>[4x]MEFKLQELNLTNQDTGPYGITVSDKGKVWITQHKANMISCINLDGKITEYPLPTPDAKVMCLTISSDGEVWFTENAANKIGRITKKGIIKEYTLPNPDSAPYGITEGPNGDIWFTEMNGNRIGRIT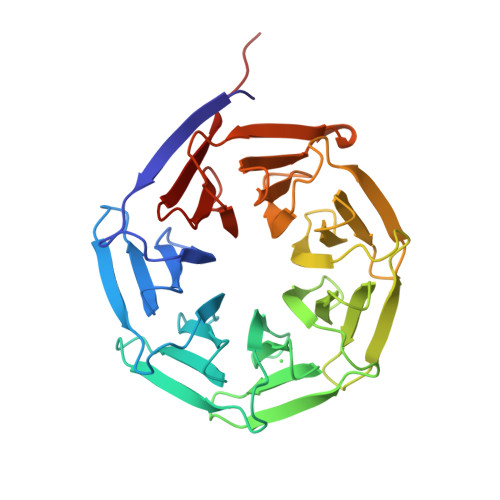DDGKIREYELPNKGSYPSFITLGSDNALWFTENQNNAIGRITESGDITEFKIPTPASGPVGITKGNDDALWFVEIIGNKIGRITTSGEITEFKIPTPNARPHAITAGAGIDLWFTEWGANKIGRLTSNNIIEEYPIQIKSAEPHGICFDGETIWFAMECDKIGKLTLIKDNME The H. pylori RNA degradosome is composed of RNase J, a 77.6 kDa enzyme that possesses both 5′−3′ exoribonuclease and endoribonuclease activities, and RhpA, a DEAD-box RNA helicase, with a molecular weight of 55.8 kDa2,7. RNase J is essential in H. pylori and plays a major role in the degradation of both mRNAs and antisense RNAs8. The central importance of RNase J in post-transcriptional regulation in H. pylori and its participation in an RNase J-based degradosome prompted us to investigate the structure, oligomeric state and post-translational regulation of the H. pylori RNase J. Here, we report the crystal and cryo-EM structures of H. pylori RNase J that assembles in tetramers organized as a dimer-of-dimers. We also show that in vitro and in solution, RNase J is in equilibrium between dimeric and tetrameric states and our data suggest that the tetrameric form constitutes the active form of RNase J in vitro.

A cryo-EM structure was obtained from purified full-length RNase J protein. The enzyme has a preferred orientation in the ice, and this has limited the resolution of the reconstructions to 4.1 angstroms. However, the reconstructions reveal unequivocally a tetrameric quaternary structure and resolve the core as well as the C-terminal oligomerization domain. The Robetta model for the CTD fits well into the map, showing good agreement with the predicted helical segments. The N-terminal region, corresponding to residues 1–136, is not resolved in the cryoEM maps. This region is not predicted to form a compact, globular structural module but rather to be intrinsically disordered. In the dimeric unit, the protomer interfaces are formed by self-complementary interactions made mostly by the CTD. The surface area buried at the CTD–CTD interface is estimated to be 1165 Å2. The beta-CASP and beta-lactamase domains of RNase J also make a self-complementary interface in the principal dimer, with an estimated area of 672 Å2 that is a little more than half of the CTD-CTD contribution. The interfaces that are formed between the dimer units to make the tetramer are also made by the beta-CASP and beta-lactamase interfaces, and these have a total buried area of 2070 Å2.

>GSGTDNNHYENNESNENSSENSKVDEARAGAFERFTNRKKRFRENAQKNGESSHHEAPSHHKKEHRPNKKPNNHHKQKHAKTRNYAKEELDSNKVEGVTEILHVNERGTLGFHKELKKGVETNNKIQVEHLNPHYKMNLNSKASVKITPLGGLGEIGGNMMVIETPKSAIVIDAGMSFPKEGLFGVDILIPDFSYLHQIKDKIAGIIITHAHEDHIGATPYLFKELQFPLYGTPLSLGLIGSKFDEHGLKKYRSYFKIVEKRCPISVGEFIIEWIHITHSIIDSSALAIQTKAGTIIHTGDFKIDHTPVDNLPTDLYRLAHYGEKGVMLLLSDSTNSHKSGTTPSESTIAPAFDTLFKEAQGRVIMSTFSSNIHRVYQAIQYGIKYNRKIAVIGRSMEKNLDIARELGYIHLPYQSFIEANEVAKYPDNEVLIVTTGSQGETMSALYRMATDEHRHISIKPNDLVIISAKAIPGNEASVSAVLNFLIKKEAKVAYQEFDNIHVSGHAAQEEQKLMLRLIKPKFFLPVHGEYNHVARHKQTAISCGVPEKNIYLMEDGDQVEVGPAFIKKVGTIKSGKSYVDNQSNLSIDTSIVQQREEVASAGVFAATIFVNKNKQALLESSQFSSLGLVGFKDEKPLIKEIQGGLEMLLKSSNAEILNNPKKLEDHTRNFIRKALFKKFRKYPAIICHAHSFGSSPHHHHHHHH[4x]>APAPATPHAPDHSPAPNSPTLTRPPEGPKFPRVKNWELGSITYDTLCAQSQQDGPCTPRRCLGSLVLPRKLQTRPSPGPPPAEQLLSQARDFINQYYSSIKRSGSQAHEERLQEVEAEVASTGTYHLRESELVFGAKQAWRNAPRCVGRIQWGKLQVFDARDCSSAQEMFTYICNHIKYATNRGNLRSAITVFPQRAPGRGDFRIWNSQLVRYAGYRQQDGSVRGDPANVEITELCIQHGWTPGNGRFDVLPLLLQAPDEAPELFVLPPELVLEVPLEHPTLEWFAALGLRWYALPAVSNMLLEIGGLEFSAAPFSGWYMSTEIGTRNLCDPHRYNILEDVAVCMDL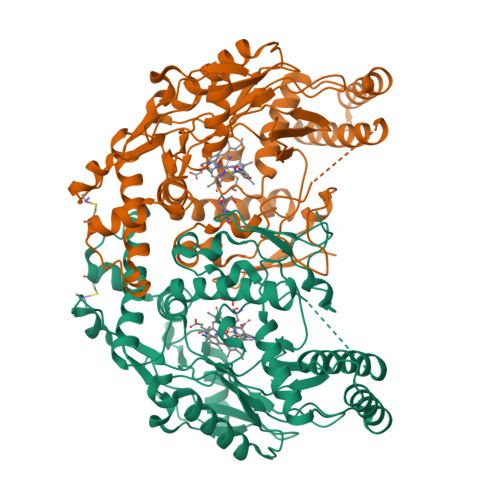DTRTTSSLWKDKAAVEINLAVLHSFQLAKVTIVDHHAATVSFMKHLDNEQKARGGCPADWAWIVPPISGSLTPVFHQEMVNYILSPAFRYQPDPW[2x]> MTAAVTPSASAVASDDKKSERRLAFWLIAPAVLLMLAVTAYPIGYAVWLSLQRYNLAEPHDTEFIGLANYVTVLTDGYWWTAFAVTLGITVVSVAIEFALGLALALVMHRTIFGKGAVRTAILIPYGIVTVAASYSWYYAWTPGTGYLANLLPEGSAPLTDQLPSLAIVVLAEVWKTTPFMALLLLAGLALVPQDLLNAAQVDGAGPWKRLTKVILPMIKPAILVALLFRTLDAFRIFDNIYILTGGSNDTGSVSILGYDNLFKAFNVGLGSAISVLIFLSVAIIAFIYIKIFGAAAPGSDEEVR;> MADRVDARRATWWSVVNILVIVYALIPVLWILSLSLKPTSSVKDGKLIPTEITFANYKAIFSGDAFTSALFNSIGIGLITTIIAVVIGGMAAYAVARLQFPGKQLLIGVALLIAMFPHISLVTPIFNMWRGIGLFDTWPGLIIPYITFALPLAIYTLSAFFREIPWDLEKAAKMDGATPAQAFRKVIAPLAAPGIVTAAILVFIFAWNDLLLA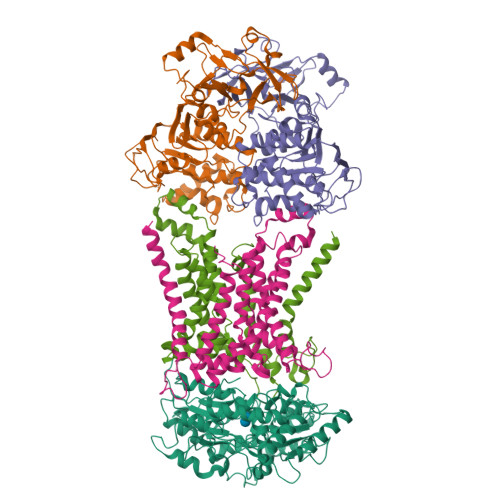LSLTATQRAITAPVAIANFTGSSQFEEPTGSIAAGAMVITIPIIIFVLIFQRRIVAGLTSGAVKG;>MAEIVLDRVTKSYPDGAGGVRAAVKEFSMTIADGEFIILVGPSGCGKSTTLNMIAGLEEITSGELRIGGERVNEKAPKDRDIAMVFQSYALYPHMTVRQNIAFPLTLAKVPKAEIAAKVEETAKILDLSELLDRKPGQLSGGQRQRVAMGRAIVRSPKAFLMDQPLSNLDAKLRVQMRAEISRLQDRLGTTTVYVTHDQTEAMTLGDRVVVMLAGEVQQIGTPDELYSSPANLFVAGFIGSPAMNFFPATRTDVGVRLPFGEVTLTPHMLDLLDKQARPENIIVGIRPEHIEDSALLDGYARIRALTFSVRADIVESLGADKYVHFTTEGAGAESAQLAELAADSGAGTNQFIARVSADSRVRTGEQIELAIDTTKLSIFDAATGLNLTRDITPTDPTEAAGPDAG[2x];> MRARRLCAAAVAAMAAASMVSACGSQTGGIVINYYTPANEEATFKAVANRCNEQLGGRFQIAQRNLPKGADDQRLQLARRLTGNDKSLDVMALDVVWTAEFAEAGWAVPLSEDPAGLAEADATENTLPGPLETARWQDELYAAPITTNTQLLWYRADLMPAPPTTWDGMLDEANRLYREGGPSWIAVQGKQYEGMVVWFNTLLQSAGGQVLSDDGQRVTLTDTPEHRAATVKALRIIKSVATAPGADPSITQTDENTARLALEQGKAALEVNWPYVLPSLLENAVKGGVSFLPLDGDPALQGSINDVGTFSPTDEQFDIAFDASKKVFGFAPYPGVNPDEPARVTLGGLNLAVASTSQHKAEAFEAIRCLRNVENQRYTSIEGGLPAVRTSLYDDPAFQKKYPQYEIIRQQLTNAAVRPATPVYQAVSTRMSATLAPISDIDPERTADELTEAVQKAIDGKGLIP> MGARALFSPHLAESALDLGVQNGTYLRGKLRVSETNCFFGEIRGQWKGHNFERVLLPGRTNLNRAIHGDIVTVELLPVASWRPLRGAKPTEEMNDTGAGGDDHENSGREGIGEESEGAALARGYTPVGRVVGITTMNRRPFCGSIDVEELNKLADTLDTLTGTVSVLFQPKDNRIPRIRITTAHLGDLKDKRLSVIIDDWGEHSSFPVGHYVEVLGTIGDKDTEAKVILLENDIPHYDFSEAVYDCLPKGEWNVTEEELGNRLDLRDLCVVSVDPLGCRDIDDALHCRRVNGNHLEVGVHIADVTHFLKEGTAMDEEAAKRSTSVYLVDRRINMLPQLLTENLCSIVADEDRYAFSIMWEFDENYSVVREFFGKTVIRSRAALYYGDAQRMIDDPEDESEAAVSLRYLMQLSRHFRKRREKDGALFLCSQEFKFKVDNDHVNPTDMQAYQTFDSNSMIEEWMLFANAAAARRVYASFPRWTLLRRHQAPAENAFDTLNEAIRRKIGVKLDDTTSLALNESLEKCVDPSDPYFNRLIRTLVTRCLRQAQYFSSSEVSKDEFHHFGLAMPIYTHFTSPIRRYADVIVHRQLAAALGIMDVSEAHMVSVKMEALASNLNYRHEQAQKAGRDSQNLFTGFYLRNFANQEIP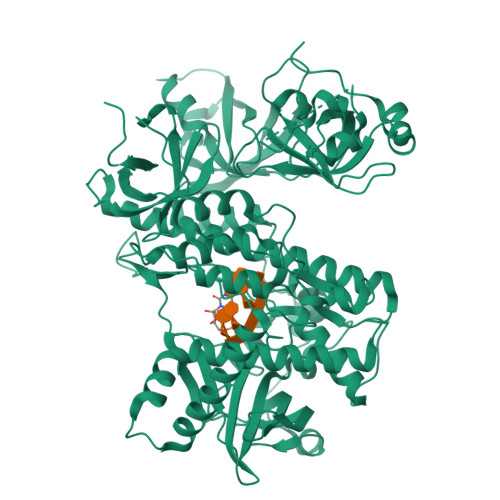SEDGYVVKLSETHVFVLVPKYGQEGKIAKETLVRVPNLLDKVKVGIEVRQRGDVLRASLVFSIIGLMKGCEDVSEPVAIAGEELPLKRQRLEHHHHHH The essential machinery responsible for the execution of apoptosis is the caspases, a family of closely related cysteine proteases. Caspases comprise two classes: the initiator caspases, such as caspase-8 and -9, and the effector caspases, such as caspases-3 and -7. For example, the autoactivation of caspase-9 is mediated by the assembly of a heptameric complex involving Apaf-1 and cytochrome c, dubbed the apoptosome. Supporting this hypothesis, caspase-9 exists predominantly as a monomer in solution and exhibits a basal level of catalytic activity.

In agreement with this analysis, previous structural investigation showed that Phe404 and Phe404′, one of the five residues on strands β6 and β6′, respectively, appear to impede the dimerization of caspase-9 by way of their incompatible side-chain configuration at the interface. To generate a potentially dimeric caspase-9, we replaced five residues in the β6 strand of caspase-9 (Gly402-Cys-Phe-Asn-Phe406) with those in caspase-3 (Cys264-Ile-Val-Ser-Met268), using standard mutagenesis methods. To solve this problem, we mutated the catalytic residue Cys287 to Ser and were able to crystallize this catalytically inactive form of the dimeric caspase-9. The structure was determined at 2.8 Å. First, the dimeric caspase-9 exists as an asymmetric homodimer in an identical manner to the WT caspase-9. Just like the WT caspase-9, there are two molecules of the dimeric caspase-9 in each asymmetric unit, and the crystal packing interaction is identical. This observation also indicates that Phe404 is not a contributing reason for the observed asymmetry in caspase-9 as previously suggested, as Phe404 is replaced by Val in the dimeric caspase-9. Second, despite being an inactive zymogen, the dimeric caspase-9 is nearly identical to the WT caspase-9 for the core structural elements, with a root mean square deviation (RMSD) of 0.4 Å over 380 aligned Cα atoms. The only significant structural difference occurs at the solvent-exposed surface loops L2, L4, L2′, and L4′. Third and most importantly, the conformation of the amino acids surrounding strands β6 and β6′ in the dimeric caspase-9 remains extremely similar or identical to that in the WT caspase-9. Thus we conclude that the impact of the five-residue replacement is naturally absorbed without any significant structural rearrangement, and that the dimeric caspase-9 faithfully mimics the dimerized state of the WT caspase-9.

>[4x]MGALESLRGNADLAYILSMEPCGHCLIINNVNFCRESGLRTRTGSNIDCEKLRRRFSSLHFMVEVKGDLTAKKMVLALLELARQDHGALDCCVVVILSHGCQASHLQFPGAVYGTDGCPVSVEKIVNIFNGTSCPSLGGKPKLFFIQASGGEQKDHGFEVASTSPEDESPGSNPEPDATPFQEGLRTFDQLDAISSLPTPSDIFVSYSTFPGFVSWRDPKSGSWYVETLDDIFEQWAHSEDLQSLLLRVANAVSVKGIYKQMPCIVSMLRKKLFFKTS3-(1~{H}-indazol-3-yl)-~{N}-[[1-(2-methylphenyl)-1,2,3-triazol-4-yl]methyl]-5-(propanoylamino)benzamide | C27 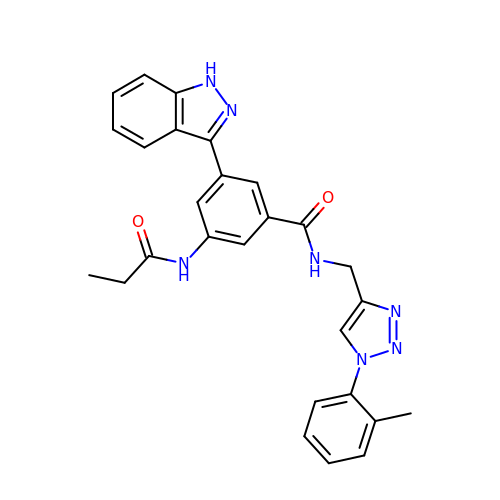H25 N7 O2 | QQDZTTUGTUHXSR-UHFFFAOYSA-N> XTIRTR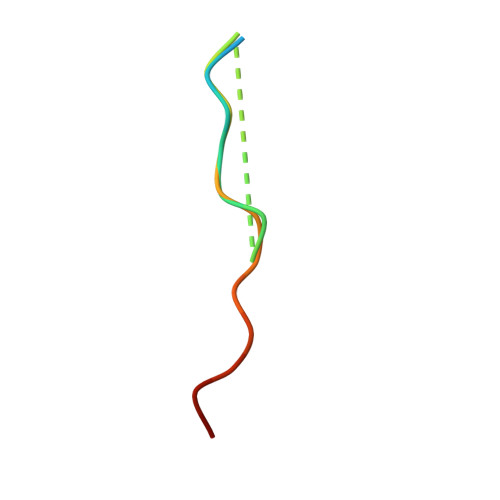GAIIQTPTLGPIQPTRX> MTRRPDRKDVATVDELHASATKLVGLDDFGTDDDNYREALGVLLDAYQGEAGLTVL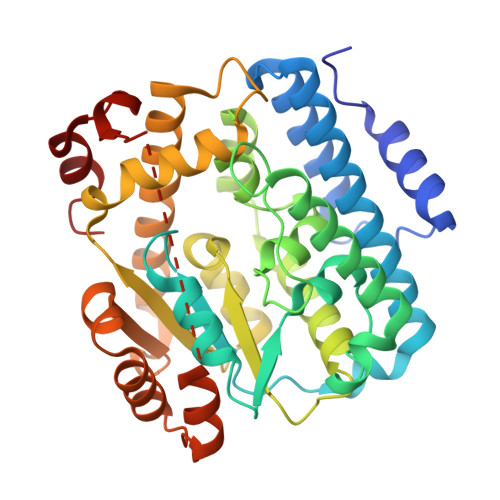GSKMNRFFLRGALVARLLSQSAWKQYPEHVDVAIKRPIFVTGLVRTGTTALHRLLGADPAHQGLHMWLAEYPQPRPPRETWESNPLYRQLDADFTQHHAENPGYTGLHFMAAYELEECWQLLRQSLHSVSYEALAHVPSYADWLSRQDWTPSYCRHRRNLQLIGLNDAEKRWVLKNPSHLFALDALMATYPDALVVQTHRPVETIMASMCSLAQHTTEGWSTKFVGAQIGADAMDTWSRGLERFNAARAKYDSAQFYDVDYHDLIADPLGTVADIYRHFGLTLSDEARQAMTTVHAESQSGARAPKHSYSLADYGLTVEMVKERFAGL>ANQPDWADEAANGAHQDAWKSLKARVENVYYMVKATYKNDPVWGNDFTCVGVMANDVNEDEKSIQAEFLFMNNADTNMQFATEKVTAVKMYGYNRENAFRYETEDGQVFTDVIAYSDDNCDVIYVPGTDGNEEGYELWT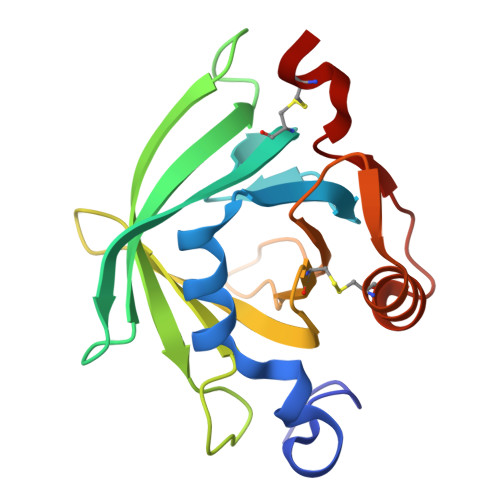TDYDNIPANCLNKFNEYAVGRETRDVFTSACLE[2x]>[12x]MTLHKERRIGRLSVLLLLNEA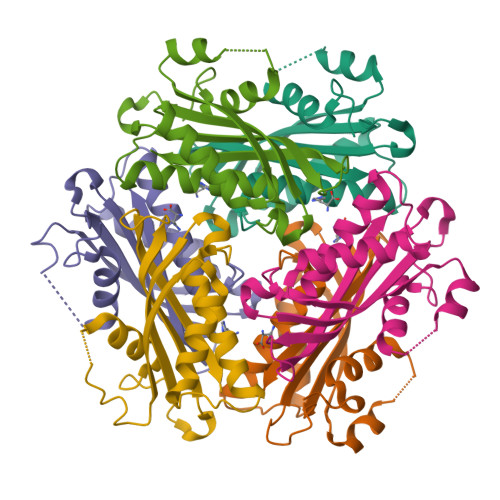EESTQVEELERDGWKVCLGKVGSMDAHKVIAAIETASKKSGVIQSEGYRESHALYHATMEALHGVTRGEMLLGSLLRTVGLRFAVLRGNPYESEAEGDWIAVSLYGTIGAPIKGLEHETFGVGINHI> GPLGSLLETKASYLCDVAGAEVVRQFLDQYFRIFDSGNRQALLDAYHEKAMLSISMPSASQAGRLNSFWKFNRNLRRLLNGEENRTRNLKYGRLACVSTLDEWPKTQHDRRTFT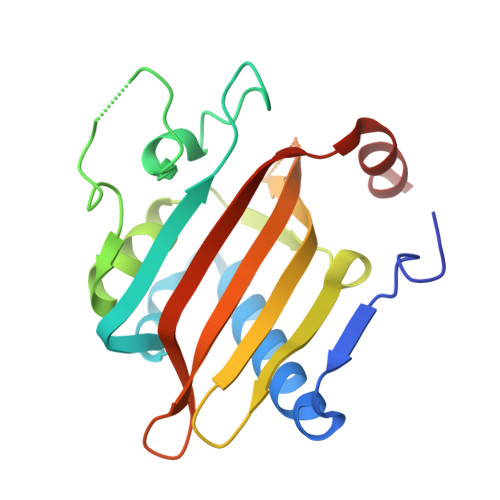VDLTIYNTSMMVFTVTGLFKELNDETNNPASMELYDVRHFARTYVVVPQNNGFCIRNETIFITNATHEQVREFKRSQ>MIQGVIQKIAGPAVIAKGMLGARMYDICKVGEEGLVGEIIRLDGDTAFVQVYEDTSGLKVGEPVVSTGLPLAVELGPGMLNGIYDGIQRPLERIREKTGIYITRGVVVHALDREKKWAWTPMVKPGDEVRGGMVLGTVPEFGFTHKILVPPDVRGRVKEVKPAGEYTVEEPVVVLEDGTELKMYHTWPVRRARPVQRKLDPNTPFLTGMRILDVLFPVAMGGTAAIPGPFGSGKTVTQQSLAKWSNADVVVYVGCGERGNEMTDVLVEFPELTDPKTGGPLMHRTVLIANTSNMPVAAREASIYVGVTIAEYFRDQGFSVALMADSTSRWAEALREISSRLEEMPAEEGYPPYLAARLAAFYERAGKVITLGGEEGAVTIVGAVSPPGGDMSEPVTQSTLRIVGAFWRLDASLAFRRHFPAINWNGSYSLFTSALDPWYRENVAEDYPELRDAISELLQREAGLQEIVQLVGPDALQDAERLVIEVGRIIREDFLQQNAYHEVDAYCSMKKAYGIMKMILAFYKEAEAAIKRGVSIDEILQLPVLERIGRARYVSEEEFPAYFEEAMKEIQGAFKALA[3x];>[3x]MDLLKKEYTGITYISGPLLFVENAKDLAYGAIVDIKDGTGRVRGGQVIEVSEEYAVIQVFEETTGLDLATTSVSLVEDVARLGVSKEMLGRRFNGIGKPIDGLPPITPEKRLPITGLPLNPVARRKPEQFIQTGISTIDVMNTLVRGQKLPIFSGSGLPANEIAAQIARQATVRPDLSGEGEKEEPFAVVFAAMGITQRELSYFIQEFERTGALSRSVLFLNKADDPTIERILTPRMALTVAEYLAFEHDYHVLVILTDMTNYCEALREIGAAREEIPGRRGYPGYMYTDLATIYERAGVVEGKKGSVTQIPILSMPDDDRTHPIPDLTGYITEGQIQLSRELHRKGIYPPIDPLPSLSRLMNNGVGKGKTREDHKQVSDQLYSAYANGVDIRKLVAIIGEDALTENDRRYLQFADAFERFFINQGQQNRSIEESLQIAWALLSMLPQGELKRISKDHIGKYYGQKLEEIWGAPQALD;> MSQVSPTRMNLLQRRGQLRLAQKGVDLLKKKRDALVAEFFGLVREAMEARKALDQAAKEAYAALLLAQAFDGPEVVAGAALGVPPLEGVEAEVENVWGSKVPRLKATFPDGALLSPVGTPAYTLEASRAFRRYAEALIRVANTETRLKKIGEEIKKTTRRVNALEQVVIPGIRAQIRFIQQVLEQREREDTFRLKRIKGKIEAREAEEEGGRPNPQVEIGAGL;> MAVIADPETAQGFRLAGLEGYGASSAEEAQSLLETLVERGGYALVAVDEALLPDPERAVERLMRGRDLPVLLPIAGLKEAFQGHDVEGYMRELVRKTIGFDIKL;>GGLGLIKSLAEKEKQLLERLEAAKKEAEERVKRAEAEAKALLEEAEAKAKALEAQYRERERAETEALLARYRERAE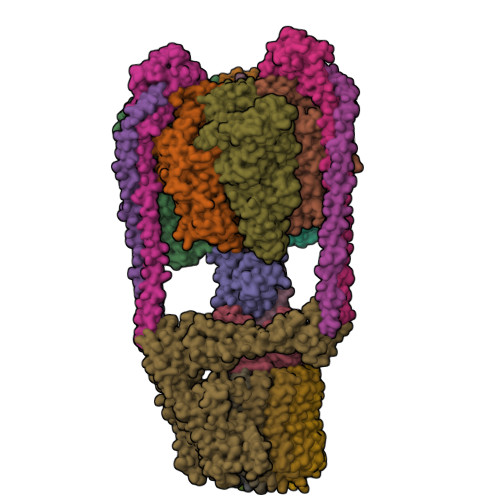AEAKAVREKAMARLDEAVALVLKEVLP[2x];>MSKLEAILSQEVEAEIQALLQEAEAKAEAVKREAEEKAKALLQARERALEAQYRAALRRAESAGELLVATARTQARGEVLEEVRRRVREALEALPQKPEWPEVVRKLALEALEALPGAKALVANPEDLPHLEALARERGVELQAEPALRLGVRAVGAEGKTQVENSLLARLDRAWDALSSKVAQALWG[2x];> MADDFAYLNARVRVRRGTLLKESFFQEALDLSFADFLRLLSETVYGGELAGQGLPDVDRAVLRTQAKLVGDLPRLVTGEAREAVRLLLLRNDLHNLQALLRAKATGRPFEEVLLLPGTLREEVWRQAYEAQDPAGMAQVLAVPGHPLARALRAVLRETQDLARVEALLAKRFFEDVAKAAKGLDQPALRDYLALEVDAENLRTAFKLQGSGLAPDAFFLKGGRFVDRVRFARLMEGDYAVLDELSGTPFSGLSGVRDLKALERGLRCVLLKEAKKGVQDPLGVGLVLAYVKEREWEAVRLRLLARRAYFGLPRAQVEEEVVCP;> MIAPMEKLVLAGPKGRAKELLQSLQQAGVVHLETLRPEALSAYQLSPEERAELRRWEAVSAGAEHTLSLLGLEAEPARPFPEGLEAAEKALSPIQAHAEGLTRQKQELEEELALAQAYLEPLERLAALAHGLDKSPFLRVIPFLLTEKELPLVEEALRKALEDRYLLAHEAYAGGVAALVVVHRKEVDQAKAALSRAGVAELRLPGALGELPLSEAARRLKERAEAAPRELSEVRQHLAKLARESASTLQSLWTRAQDEVARLKALEELASGRFGFALLGYVPVKAKPKVEEALARHKESVVYAFEPVDEHHEADRIPVVLDNPPWAKPFELLVSFLNTPKYGTFDPTPVVPVFFPFWFGMIVGDIGYALLFYLVGRWLSGYVKRNEPLVIDLFALKLKPQVIGKLVHILNWMVFWTVVWGVIYGEFFGTFLEHLGVFGTPEHPGLIPILIHRIDTAKTANLLILLSVAFGVVLVFFGLALRAYLGLKHRHMAHFWEGVGYLGGLVGVLALAASYLGNLQAGWLQGLMYLGFGVFLLAVLMSRIWLMIPEIFTQAGHILSHIRIYAVGAAGGILAGLLTDVGFALAERLGLLGVLLGLLVAGVLHLLILLLTTLGHMLQPIRLLWVEFFTKFGFYEENGRPYRPFKSVREAQ;>SGGLDRGLIAVGMGLAVGLAALGTGVAQARIGAAGVGAIAEDRSNFGTALIFLLLPETLVIFGLLIAFILNGRL[12x]Na+/H+ exchangers facilitate the exchange of monovalent cations (Na+/Li+/K+) and protons (H+) across membranes to regulate intracellular pH, sodium levels and cell volume. Na+/H+ exchangers that perform this task are physiological homodimers, and whilst the ion transporting domain is highly conserved, their dimerization differs. The transporter is made up of two distinct domains, a dimerization domain and an ion-transporting (core) domain. Here, we report cryo-EM structures of E. coli NhaA and E. caballus NHE9 in complex with cardiolipin and phosphatidylinositol-3,5-bisphosphate PI(3,5)P2 lipids binding at their respective dimer interfaces.

Here, we instead performed the collection of NHE9* at pH 6.5 where NHE9 is thought to be less active, and therefore presumably less dynamic. Overall, we collected ~4300 movies and the final 3D-reconstruction contained data of ~244,300 particles, from which an EM map could be reconstructed to 3.3 Å according to the gold-standard Fourier shell correlation (FSC) 0.143 criterion. Selecting 42% of the particles for heterogeneous refinement, enabled an improved cryo-EM map reconstruction of NHE9* at pH 6.5, with additional map features for the TM2-TM3 loop domain. For model building we therefore generated a composite map, by combining the maps before and after masked refinement, with an overall resolution estimate of 3.6 Å, although the final model resolution is worse at 4.0 Å resolution. We were able to refine the overall position of the short linker and β-hairpin strand predicted from the AlphaFold228 model. The loop domain reconnects to the beginning of TM3 via a short extracellular helix (ECH1), which was well supported by the cryo-EM maps. The β-hairpins were predicted by AlphaFold228 to be domain-swapped, and this structure refines well into the map density. The centre of the loop domain has a cluster of positively-charged residues K105, K107 and R108 from each of the two protomers. Overall, the TM2-TM3 β-loop domain clasps the two protomers together on the luminal side and forms a highly positively-charged cluster that is positioned above the dimerization domain interface. As such, the improved NHE9* structure is consistent with its previously proposed requirement for binding negatively-charged PIP2 lipids at the interface.

>[2x]MSEKDEYQFQHQGAVELLVFNFLLILTILTIWLFKNHRFRFLHETGGAMVYGLIMGLILRYATAPTDIESGTVYDCGKLAFSPSTLLINITDQVYEYKYKREISQHNINPHLGNAILEKMTFDPEIFFNVLLPPIIFHAGYSLKKRHFFQNLGSILTYAFLGTAISCIVIGLIMYGFVKAMVYAGQLKNGDFHFTDCLFFGSLMSATDPVTVLAIFHELHVDPDLYTLLFGESVLNDAVAIVLTYSISIYSPKENPNAFDAAAFFQSVGNFLGIFAGSFAMGSAYAVVTALLTKFTKLCEFPMLETGLFFLLSWSAFLSAEAAGLTGIVAVLFCGVTQAHYTYNNLSLDSKMRTKQLFEFMNFLAENVIFCYMGLALFTFQNHIFNALFILGAFLAIFVARACNIYPLSFLLNLGRKHKIPWNFQHMMMFSGLRGAIAFALAIRDTESQPKQMMFSTTLLLVFFTVWVFGGGTTPMLTWLQIRVGVDLDEDLKERPSSHQEANNLEKSTTKTESAWLFRMWYGFDHKYLKPILTHSGPPLTTTLPEWCGPISRLLTSPQAYGEQLKEGENLYFQ> MQNALKVGFWPAYSVSEFPPSKINSRLFTHLYYAFAELNAPTFEVRVPPGSEKTAEDFTPTVRRLNPSVKTLISIGGGGSEVRDNFAKLNSDASARQRFVKSSIALARRYGFHGLDLDYQYPEPQLEMENFVKLVSELTAAIREEARTSGKPRLLLTEAVYFHQKLFPWEVVTEYPVQFIAAG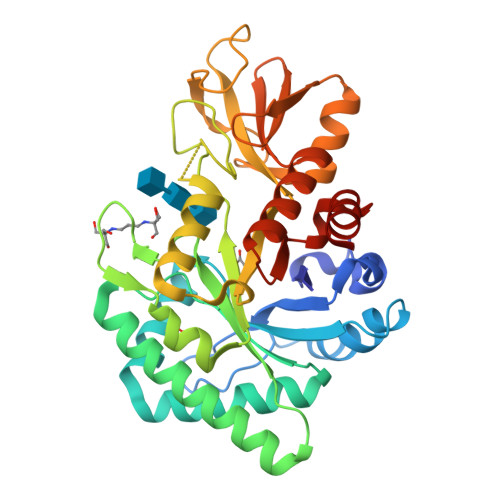LDWVNVMAYDFHGSWENFTGAPAALRDPNSKFTASVGIESFLAAGMPPEKLVLGIPLFGRSWLLKNNNEVGIGAPAVGAGPVDGALSFSEIQNFIRGGAREVFDTTTVSAYAYKDNVWVGYDNQQSVALKVQYAKEKRLGGYFFWSVNQDIDAILPKIASDTWGG>GPGTMMNVIMREIGKKLD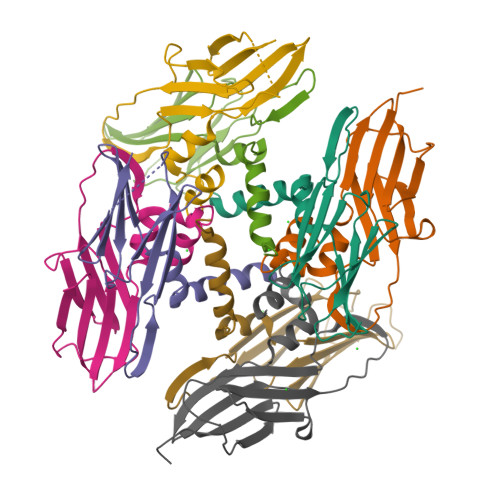ELSREFYESVIPPIDMYEEGGELVVVADLAGFNKDKISVRLSAQNELIINAEREIQYIGTKYATQRPLKIHKVIRLPVKVKRDSQVTAKYENGVLTIRIPVEGSVS[8x]The DNA resolvases orthologous to the A22 protein of vaccinia virus play an essential role in poxviral replication, by resolving HJ structures formed at the inverted repeat junctions in a concatemer of linear genomic DNAs. The poxvirus resolvases belong to the RNaseH/retroviral integrase superfamily of DNA-modifying enzymes that employ a conserved metal-dependent mechanism, including the prototypical bacterial RuvC HJ DNA resolvase. The fowlpox virus resolvase (Fpr) forms a stable dimer as other homologous resolvases14–17 and was found to bind to various structural motifs on the HJ DNA, revealing flexibility of the Fpr dimer in binding to a wide range of DNA structures. The 150-residue Fpr protein has the characteristic architecture of enzymes from the retrovirus integrase/RNase H superfamily, comprising a single layer of β-sheet sandwiched between α-helices.

Initial crystallization of C151stop Fpr with a catalytic mutation D135N to abolish the nuclease activity, in the presence of a HJ DNA yielded large crystals that diffracted only up to 7~8 Å resolution. Four additional surface conformational entropy reduction mutations, K65A, K102A, K103A, and Q104A, helped improve crystal quality and the structure was determined and refined to 3.1 Å. A HJ DNA substrate, HJ 13/13 with four 13 bp arms, was required for crystallization of Fpr and present in the washed crystals. However, no DNA molecules were observed in the electron density map and the structure obtained was that of Fpr in the APO (DNA-free) form. Divalent cadmium ion used in the crystallization reservoir solution at 10 mM concentration, was identified in the active center pocket, coordinated by the acidic active site residues, D7, E60, D132, and N135 (D135 in the wild-type). In the Fpr dimer, αB helices from each protomer form the major dimer interface. The dimer interface is mainly formed by the hydrophobic interactions, including F64, Y73, F74, F78, and Y80. A notable difference is that the Cpr crystal structure does not have clear electron density for the helix αD, whereas the Fpr structure shows a well ordered αD helix with clear electron density. In contrast, the active sites and the surrounding DNA-binding surfaces of the two Fpr monomers are not well separated due to the shorter αB and the loop preceding the αB helix, and they form a larger flat pocket.

>[2x]MIICSVDIGIKNPAYAIFNYDNTSNTIKLIAIEKSDWTKNWERSVARDLTRYNPDVVILEKQGFASPNSKIIYFIKGFFYNSNTKVIVRNPTFKGGSYRNRAAASIDVFIQKISEYTDYKNDILNKYTKLDDIANSFNLGLSYMESLL Glutathione transferases (GSTs, EC 2.5.1.18) comprise a family of widely distributed phase II detoxification enzymes that catalyze the conjugation of a broad variety of reactive electrophiles to the nucleophilic sulfur atom of the intracellular thiol, tripeptide glutathione (γ-L-Glu-L-Cys-Gly). Each subunit contains an active site that consists of a GSH-binding site (G-site) in the N-terminal domain and a site that binds the hydrophobic substrate (H-site) in the C-terminal domain. Moreover, the isoenzyme GSTM1-1 is mostly studied in humans for its correlation with many types of cancer, while other studies support its pertinence with Parkinson’s disease. The present study aims to evaluate the ligandability of the human GSTM1-1 isoenzyme (hGSTM1-1) using a broad range of structurally diverse pesticides as probes.

To shine a light on the restricted hGSTM1-1 ligand-binding promiscuity, the ligand-free crystal structure of hGSTM1-1 was determined by X-ray crystallography at 1.59 Å-resolution. The enzyme was crystallized in the P21 space group resulting in four molecules (A, B, C, D) in the asymmetric unit. D–A and C–B form the typical dimers found in GSTs. The interface area of D–A and C–B dimers is 1341.9 Å2 and 1313.1 Å2, respectively. The interactions between dimers are mediated through helix α7 (residues 178–189). The most noticeable difference was observed in Arg42, which is involved in the formation of a salt bridge with GSH and points closer to the active site cavity in the high-resolution hGSTM1 structure than in its low-resolution counterpart. Indeed, the cavity volume for the ligand-free hGSTM1-1 is ~8.6 Å3, for the GSH-bound enzyme it is ~32.4 Å3 and for the GSH-CDNB conjugate the cavity volume is ~55.7 Å3. Since co-crystallization of enzyme/pirimicarb was not achieved due to the high-salt condition in the crystallization medium, a molecular-docking study was carried out, taking advantage of the high-resolution structure reported here. The compound binds to the enzyme at a distinct site that partially overlaps with the H-site.

>MPMILGYWDIRGLAHAIRLLLEYTDSSYEEKKYTMGDAPDYDRSQWLNEKFKLGLDFPNLPYLIDGAHKITQSNAILCYIARKHNLCGETEEEKIRVDILENQTMDNHMQLGMICYNPEFEKLKPKYLEELPEKLKLYSEFLGKRPWFAGNKITFVDFLVYDVLDLHRIFEPKCLDAFPNLKDFISRFEGLEKISAYMKSSRFLPRPVFSKMAVWGNK[4x]>[4x]MIIYRDLISHDVMFSDIYKIREIADGLCLEVEGKMVSRTEG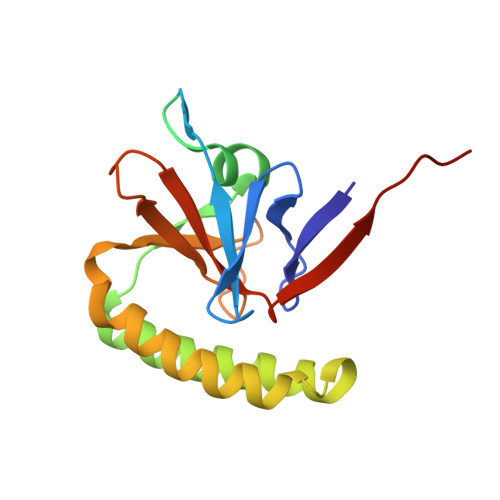NIDDSLIGGNASAEGPEGEGTESTVITGVDIVMNHHLQETSFTKEAYKKYIKDYMKSIKGKLEEQRPERVKPFMTGAAEQIKHILANFKNYQFFIGENMNPDGMVALLDYREDGVTPYMIFFKDGLEMEKCLEHHHHHH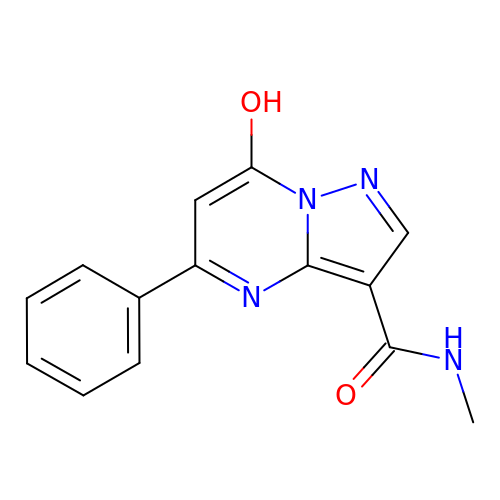7-hydroxy-N-methyl-5-phenylpyrazolo[1,5-a]pyrimidine-3-carboxamide | C14 H12 N4 O2 | RUSORFYZKCLNDR-UHFFFAOYSA-N> SNAMSQQVTQLNPTQQTTQSAFLATTVITAQCHAILNTQFTPPTVKPDWFDDLSKKLDSAKLVAKQWIDDLGPQVSASIPSSVINFDATFQASIDAI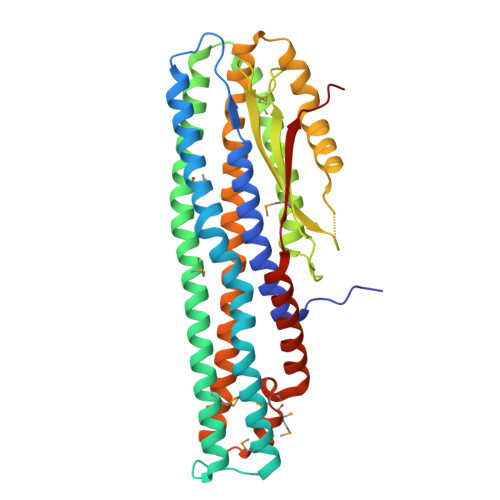HELYKADPTASGKDNTTVQQASQIMTALSSQVSGIEATVKGMNKELSDWGVKMQAAHDDLVNGATNIQKTIIDLQTDIESMNNAIDNNRAAIEKLNKDLVYAQVAVGVGIFMLVAGVALTVATAGTAAAVSGGIAAVGAASIIAGGVTWGVLQNQIDDDYDSIAQEQKQKAEDQQQIIALQGLSNASSAVVSAIETSTSVLSDFETTWTVFGNELDDVVTKLNNGASMQSIIMEKVMSDAAKNEWDDAVELAKQLASAKIAIETKELAPAVKQAA Mycobacterium tuberculosis (Mtb) WhiB3 is an iron–sulfur cluster-containing transcription factor belonging to a subclass of the WhiB-Like (Wbl) family that is widely distributed in the phylum Actinobacteria. WhiB3 plays a crucial role in the survival and pathogenesis of Mtb. It binds to the conserved region 4 of the principal sigma factor (σA4) in the RNA polymerase holoenzyme to regulate gene expression like other known Wbl proteins in Mtb. Here we determined crystal structures of the WhiB3:σA4 complex without and with DNA at 1.5 Å and 2.45 Å, respectively, to elucidate how WhiB3 interacts with DNA to regulate gene expression. These structures reveal that the WhiB3:σA4 complex shares a molecular interface similar to other structurally characterized Wbl proteins and also possesses a subclass-specific Arg-rich DNA-binding motif.

We also generated a truncated WhiB3, denoted WhiB3TR, without the C-terminal residues (aa 91–102) containing the putative DNA binding motif to improve the protein stability and crystallizability. Two crystal forms were observed from the same crystallization drop, with the larger crystals in the P43212 form and the small ones in the R3 form. However, in the crystals, the His6-tags in the N-terminal σA4-βtip of three WhiB3:σA4-βtip complexes are “glued” together by multiple nickel ions from the crystallization solution, resulting in a trimer of the WhiB3:σA4-βtip complexes in both crystal forms. Three WhiB3:σA4-βtip complexes in the trimer form are found in the asymmetric unit of the P43212 structure. The crystal structures of the WhiB3:σA4-βtip complex in the P43212 and R3 forms are essentially identical except for the N-terminal loop region, with an average Cα root-mean-square deviation of 0.27 Å for WhiB3 and 0.42 Å for σA4, respectively. First, the N-terminal residues (aa 446–456) of σA4 in the WhiB3:σA4-βtip trimer form a β-hairpin with the His6-tag residues, instead of being part of helix hs1 of σA4 as expected. Because the residues 446 to 456 of σA4 are far from the WhiB3 binding site, we do not anticipate this structural change affects the mode of WhiB3 binding to σA4. Second, βtip in the WhiB3:σA4-βtip complex, which was expected to form intramolecular contacts with σA4 in the σA4-βtip chimera, sticks into a neighboring protomer of the trimer and forms intermolecular interactions with σA4 in a second WhiB3:σA4-βtip complex. The resulting σA4-βtipʹ, however, resembles σA4-βtip observed in the WhiB7:σA4-βtip complex and the RNAP holoenzyme, and thus it is used for the following structural analysis.

>[3x]MPQPEQLPGPNADIWNWQLQGLCRGMDSSMFFHPDGERGRARTQREQRAKEMCRRCPVIEACRSHALEVGEPYGVWGGLSESERDLLLKG;>MAHHHHHHVAVDAVSFTLLQDQLQSVLDTLSEREAGVVRLRFGLTDGQPRTLDEIGQVYGVTRERIRQIESKTMSKLRHPSRSQVLRDYLDGSSGSGTPEERLLRAIFGEKA[3x]> MAAAESHMTSFQAEDWAGSNILPMVQRAGGSTRGIMAASVNLERSYMELIGAERETSRRNFRDLSLRPDVSLVIGGPKYSDCAGGYCYNESGSLLSATRNRFIHWTSYADTLELVELSLDINLLNNAVRLKILNCSILPGGVHICETQNNIIVLILTNQTVHRLILPHPSRMYRSEIISDSHIQSIFTDIGKTNFHDPNNTYVIPAIPGRAPNSTASTAWLSSDGEALFALPSVSGGILVIKMPPRDMEGLVTIAELKQSSVMQRLLTGWMPSSIRGDPGPAHLPVSLAVHTLDHDSYLFALCQDHKLRMWSYKDQMCLMVADMLEYVPVSKDIRQTAGTGHKLRLAYSDTLEILYLGVYLHTPRQGQFCVFQLVCTESNRYSLEHTSSIFTNQETLIDFTFTLSSMNIWALWLDDDNQTVMKHINFERNQAGHWNPVFVNPLPDDDLAIGDEQEPQEAYLECLFAPGRFTIAALQKAIQILRKGSGRVLDLSWEELKKEVTLTVEKEIQNAVVDYDVSQEEFRQINIENWCKFYTCCLQYQETLSRPLALVVHPNTNMVCLLRKGFLSFLAPCSSVEHLYLVPGEHLLTVDESVICDDVDGASDIVSLIQCLHMIADYITEDMAYQMESACCHPQSPERVAEQILEDLIANDIDNIMENIQNKLQDIRNPIQAISFLLQNMDYETNMDMEQSQHNVRLNLSTLYGSVTASS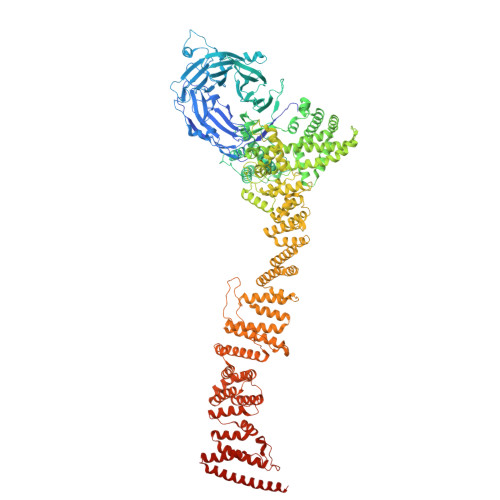VVCQAIYKISATRFLICRDLLILQHLLLRLGDMALVGAGQLLHSQQELIPRAAQLLLSYYMIRWGSQCLACAVPVDLLESNLQHLSVLELSDSQVEKRRYTSGIQTIVELFFEDVGRKHFPQVFAHLFIQSGSSQVHRSLNWADLIHRITSYLLQLLWPSNPNFQFAECLMRNCQYTQLQEYVRLLLPWCQVNVGSCHFMLAQCYLVAGEGHKALDCFSQAASEVEREDFLEKLIRVEEGESVSPRLQYYNRVLRLLEDVGLPELVIQLATIAISEASDDWRSQAALRTRIFKHHLDMGHNSQAYDALTQIPDTSRQLDCLRQLVVVLCERSQLQDLVEFPYVNLHNEVVGIIESRARAVDLMTHNYYELLYAFHIYRHNYRKAGTVMFEYGMRLGREVRTLRGLQKQVNSYLACLNCLRLIRPEYAWIVQPVSGAVYERPGASPKRNYDGESSAVPSSSQIEILELRDLEKEYVLAQTRLTLAKHNPSTAAIAGSSAAEEMVALLVQAGLFDTAISLCQTFKLGLTSIFEGLACKCIRLQQGGEAAQAEAWEWLAANQLATVITTKESSATDEAWRLMISYLDKYESKNTLYHHCIINKLLSHGVPLPNWLINRYKAMDAAELLRLYLKYDLLEEAAELVLEYVDALLGKGHQYFGIQAPLSATSQLVWFPYSAIDHLRLALGENENNQHNQAILGKLQRKMDEYFQKLKKATDDYKKIVQKPVRA2-azanyl-7,8-dihydro-6~{H}-quinazolin-5-one 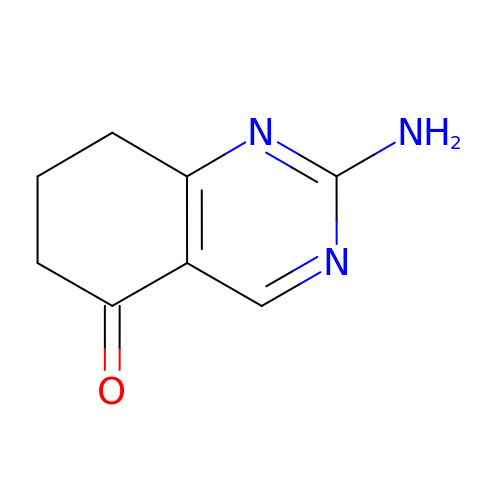| C8 H9 N3 O | ZXWJMLMXKMSYTP-UHFFFAOYSA-N> GSMLSAFTARPIIELKPRDKSRIECILAYGDRVLVGLNTGSLRVYRVNDLSPSPSPANPSDSQSPEASQSSVNPDPSSSTQDPSSQPDSQPVVPQQKPTDLLREIERFSPRAIEQLAIIKEANTLVSLSNYCVSLHDLHTFEPIASPLPRTKNASGFAVTSNIVKDPATGIPEIISRLAVSVKRRLLLWSWHESELEEEVKEVVLTESIRSMTWACATRLVCGMNSGFVVVDVETGTVEDILGPPGGAAGGNQGRWGAVSAGGMGYMGLGGYMPKPLCTKLADGQLLLAKDVNTLFIDDTGKALEKRQIPWQAAPDGIGYSYPYILALQPPAKGCLEVRNPDTLSLLQTLSLPGAAALHFPPPTVSLAHAGKGFHVLSDRVVWKMDATDYDSQVEELVRGGKLDEAISVLTMLEDALLKNKTETLREVKMQKAEVLFRQKKYRESMDLFNEDEVNAPPERVLRLFPKSIAGELSGVEEEKQGQSQQSDSEQEGSSNGTATAD

Lysosomal fusion is fundamental to cell survival and requires HOPS, a conserved heterohexameric tethering complex. The heterohexameric HOPS complex mediates fusion of late endosomes, autophagosomes, and AP-3 vesicles with mammalian lysosomes or vacuoles in yeast, and is probably the best-studied tethering complex. Five out of six HOPS subunits (Vps11, Vps16, Vps18, Vps39, and Vps41) are predicted to share a similar architecture, comprising an N-terminal β-propeller and a C-terminal α-solenoid domain. At the opposite sites, Vps41 and Vps39 bind to membrane-anchored small GTPases (the Rab7-like Ypt7 in yeast), while Vps16 and the SM protein Vps33 establish the SNARE-binding module.

To address this, we first analyzed the N-terminal β-propellers of Vps41 and Vps39, the likely binding sites with Ypt7. The intrinsic low affinity between HOPS and Ypt7 prevented reconstitution of the complex for structural studies, therefore, we instead relied on AlphaFold predictions. Additionally, we solved the structure of the β-propeller of Chaetomium thermophilum Vps39 by X-ray crystallography, which largely confirmed the predicted model. Cristal structure of C. thermophilum Vps39 (1–500) construct (cyan) is shown and superimposed on the model of Saccharomyces cerevisiae Vps39 (dark green) generated by AlphaFold. Surprisingly, in the AlphaFold model, Ypt7 binding occurs at the α-solenoid of Vps39 where it does not directly interact with the β-propeller, as originally expected. Furthermore, the binding site on Vps39 is placed approximately 5–6 nm above the membrane if Ypt7-anchored HOPS is in an upright position on supported lipid bilayers. Membrane-bound Ypt7 can still reach this site due to its 10 nm long hypervariable domain (not shown in the prediction).> ATITQDTPINQIFTDTALAEKMKTVLGKTNVTDTVSQTDLDQVTTLQADRLGIKSIDGVEYLNNLTQINFSNNQLTDITPLKNLTKLVDILMNNNQIADITPLANLTNLTGLTLFNNQITDIDPLKNLTNLNRLELSSNTISDISALSGLTSLQQLNFSSNQVTDLKPLANLTTLERLDISSNKVSDISVLAKLTNLESLIATNNQISDITPLGILTNLDELSLNGNQLKDIGTLASLTNLTDLDLANNQISNLAPLSGLTKLTELKLGANQISNISPLAGLTALTNLELNENQLEDISPISNLKNLTYLTLYFNNISDISPVSSLTKLQRLFFYNNKVSDVSSLANLTNINWLSAGHNQISDLTPLANLTRITQLGLNDQAWTNAPVNYKANVSIPNTVKNV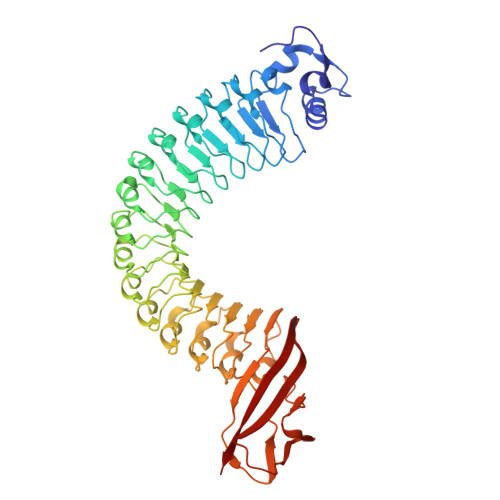TGALIAPATISDGGSYTEPDITWNLPSYTNEVSYTFSQPVTIGKGTTTFSGTVTQPLKA> GTTAK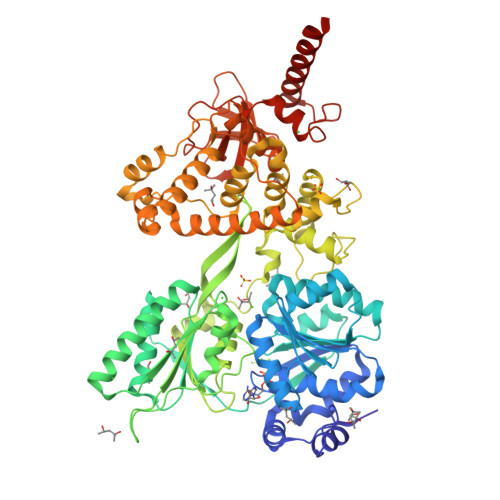QAEAVEDSDINPWTGQRHSERYFKILKARRKLPVNKQRQEFLDLYHNNQILVFVGETGSGKTTQIPQYVLYDELPHQTGKLIACTQPRRVAAMSVAQRVADELDVKLGEEVGYSIRFENKTSSKTLLKYMTDGQLLREAMHDRDMSRYSCIILDEAHERTLATDILMALLKQLSERRKDLKIIVMSATLDAQKFQSYFFNAPLLAVPGRTHPVEIFYTPEAERDYVEAAIRTVLQIHACEPEGDILLFLTGEEEIEDACRRISLEVDEMIRESDAGPMSVYPLYGTLPPHQQQRIFEKAPQPFRPGGRPGRKCIVATNIAETALTIDGIVYVVDPGFSKQKIYNPRTRVESLLVSPISKASAQQRAGRAGRTRPGKCFRLYTEEAFKKELIEQTYPEILRSNLSNTVLELKKLGVEDLVHFDLMDPPAPETMMRALEELNYLACLDDDGELTPLGNLASEFPLDPALAVMLISSPEFYCSNEILSITSLLSVPQIWVRPANARKRADEMKAQFAHPDGDHLTLLNAYHAYKGAEARGEDMKKWCHEHFLSYRHLSSADNVRAQLKKIMETHGIELVSTPFHDKNYYTNIRRALLAGFFMQVAMRESSNSKVYKTVKDEQLVLIHPSTTVTTPYEWVVYNEFVLTTKQYVRTVTNIRPEWLLEIAPVYYDLSTFQKGEIKNALTRVAEKIRRQQAMKASKA> MGHHHHHHAENLYFQGAPFESYNPEFFLYDIFLKFCLKYIDGEICHDLFLLLGKYNILPYDTSNDSIYACTNIKHLDFINPFGVAAGFDKNGVCIDSILKLGFSFIEIGTITPRGQTGNAKPRIFRDVES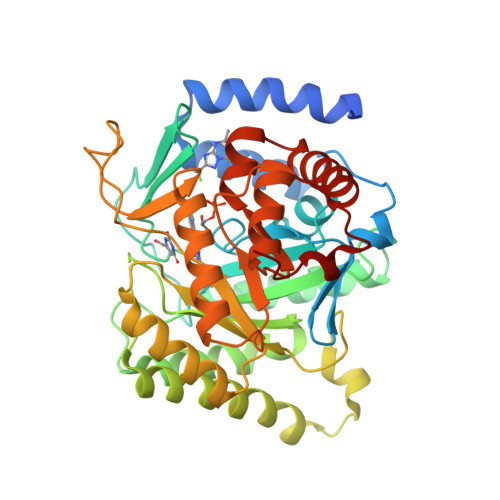RSIINSCGFNNMGCDKVTENLILFRKRQEEDKLLSKHIVGVSIGKNKDTVNIVDDLKYCINKIGRYADYIAINVSSPNTPGLRDNQEAGKLKNIILSVKEEIDNLEKNNIMNDEFLWFNTTKKKPLVFVKLAPDLNQEQKKEIADVLLETNIDGMIISNTTTQINDIKSFENKKGGVSGAKLKDISTKFICEMYNYTNKQIPIIASGGIFSGLDALEKIEAGASVCQLYSCLVFNGMKSAVQIKRELNHLLYQRGYYNLKEAIGRKHSKS> GLIVDTRDVEERVHVMRKTKLAPTVAHGVFNPEFGPAALSNKDPRLNEGVVLDEVIFSKHKGDTKMSAEDKALFRRCAADYASRL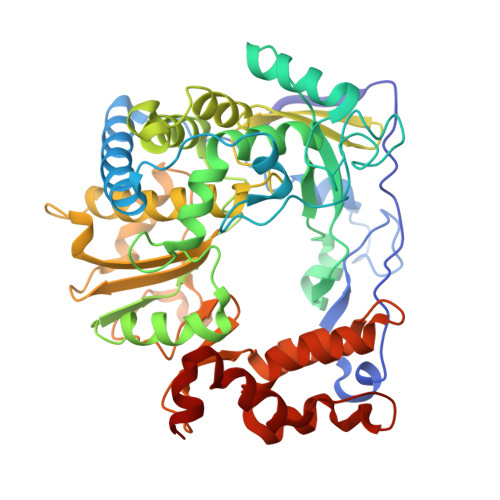HSVLGTANAPLSIYEAIKGVDGLDAMEPDTAPGLPWALQGKRRGALIDFENGTVGPEVEAALKLMEKREYKFACQTFLKDEIRPMEKVRAGKTRIVDVLPVEHILYTRMMIGRFCAQMHSNNGPQIGSAVGCNPDVDWQRFGTHFAQYRNVWDVDYSAFDANHCSDAMNIMFEEVFRTEFGFHPNAEWILKTLVNTEHAYENKRITVEGGMPSGCSATSIINTILNNIYVLYALRRHYEGVELDTYTMISYGDDIVVASDYDLDFEALKPHFKSLGQTITPADKSDKGFVLGHSITDVTFLKRHFHMDYGTGFYKPVMASKTLEAILSFARRGTIQEKLISVAGLAVHSGPDEYRRLFEPFQGLFEIPSYRSLYLRWVNAVCGDAAALE>[2x]MENTENSVDSKSIKNLEPKIIHGSESMDSGISLDNSYKMDYPEMGLCIIINNKNFHKSTGMTSRSGTDVDAANLRETFRNLKYEV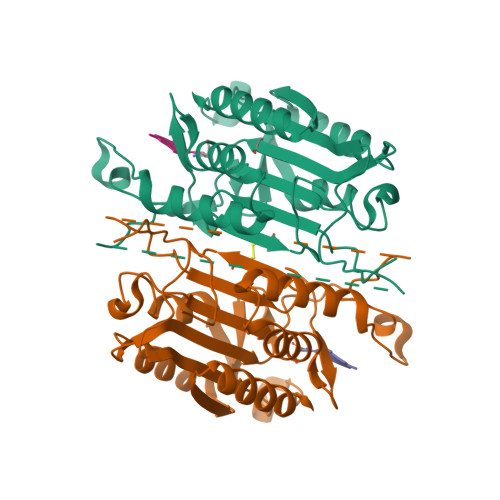RNKNDLTREEIVELMRDVSKEDHSKRSSFVCVLLSHGEEGIIFGTNGPVDLKKITNFFRGDRCRSLTGKPKLFIIQACRGTELDCGIETDSGVDDDMACHKIPVEADFLYAYSTAPGYYSWRNSKDGSWFIQSLCAMLKQYADKLEFMHILTRVNRKVATEFESFSFDATFHAKKQIPCICSMLTKELYFYHL>[2x]PNFSGNWKIIRSENFEELLKVLGVNVMLRKIAVAAASKPAVEIKQEGDTFYIKVSTTVRTTEINFKVGEEFEEQTVDGRPCKSLV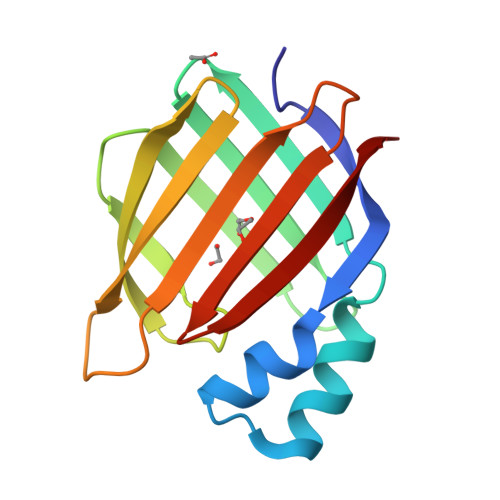KWESENKMVCEQKLLKGEGPKTSWTLELTNDGELIDTMTADDVVCTKVFVRE> GPDSMADAFGDELFSVFEGDSTTAAGTKKDKEKDKGKWKGPPGSADKAGKRFDGKLQSESTNNGKNKRDVDFEGTDEPIFGKKPRIEESITEDLSLADLMPRVKVQSVETVEGCTHEVALPAEEDYLPLKPRVGKAAKEYPFILDAFQREAIQCVDNNQSVLVSAHTSAGKTVCAEYAIALALREKQRVIFTSPIKALSNQKYREMYEEFQDVGLMTGDVTINPTASCLVMTTEILRSMLYRGSEVMREVAWVIFDEIHYMRDSERGVVWEETIILLPDNVHYVFLSATIPNARQFAEWICHLHKQPCHVIYTDYRPTPLQHYIFPAGGDGLHLVVDENGDFREDNFNTAMQVLRDAGDLAKGDQKGRKGGTKGPSNVFKIVKMIMERNFQPVIIFSFSKKDCEAYALQMTKLDFNTDEEKKMVEEVFSNAIDCLSDEDKKLPQVEHVLPLLKRGIGIHHGGLLPILKETIEILFSEGLIKALFATETFAMGINMPARTVLFTNARKFDGKDFRWISSGEYIQMSGRAGRRGMDDRGIVILMVDEKMSPTIGKQLLKGSADPLNSAFHLTYNMVLNLLRVEEINPEYMLEKSFYQFQHYRAIP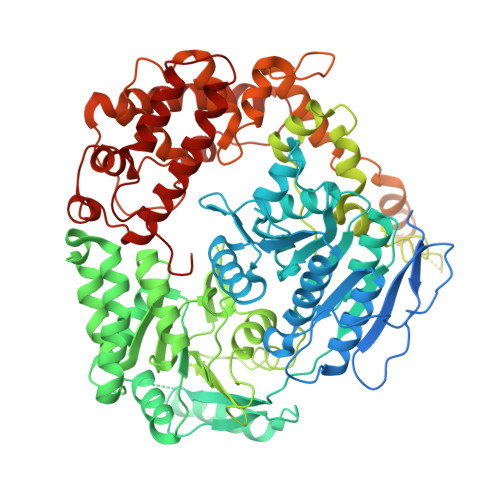GVVEKVKNSEEQYNKIVIPNEESVVIYYKIRQQLAKLGKEIEEYIHKPKYCLPFLQPGRLVKVKNEGDDFGWGVVVNFSKKSNVKPNSGELDPLYVVEVLLRCSKESLKNSATEAAKPAKPDEKGEMQVVPVLVHLLSAISSVRLYIPKDLRPVDNRQSVLKSIQEVQKRFPDGIPLLDPIDDMGIQDQGLKKVIQKVEAFEHRMYSHPLHNDPNLETVYTLCEKKAQIAIDIKSAKRELKKARTVLQMDELKCRKRVLRRLGFATSSDVIEMKGRVACEISSADELLLTEMMFNGLFNDLSAEQATALLSCFVFQENSSEMPKLTEQLAGPLRQMQECAKRIAKVSAEAKLEIDEETYLSSFKPHLMDVVYTWATGATFAHICKMTDVFEGSIIRCMRRLEELLRQMCQAAKAIGNTELENKFAEGITKIKRDIVFAASLYL> MNVGDRVRVTSSVVVYHHPEHKKTAFDLQGMEGEVAAVLTEWQGRPISANLPVLVKFEQRF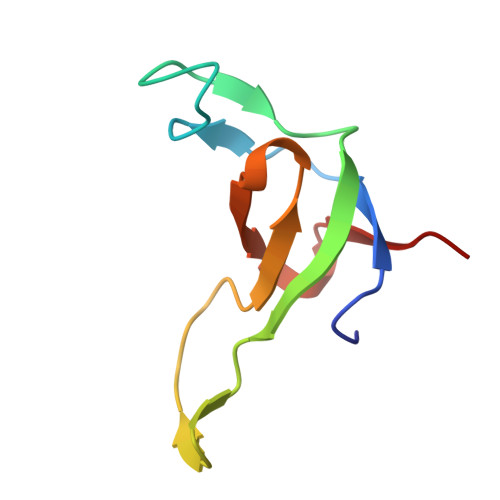KAHFRPDEVTLIE> MHHHHHHGENLYFQGSGVEVIFYLSDREPLRLGSGEYTAEELCIRAAQACRISPLCHNLFALYDEN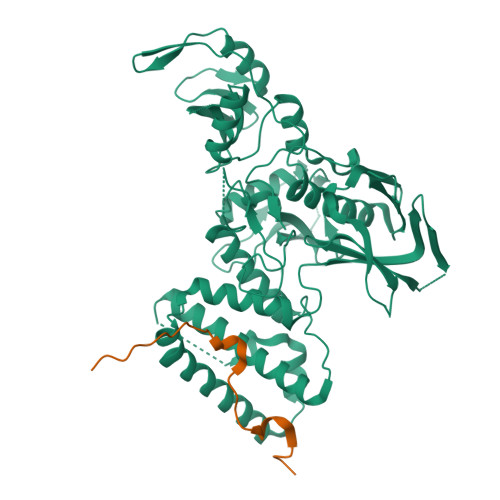TKLWYAPNRTITVDDKMSLRLHYRMRFYFTNWHGTNDNEQSVWRHSPKKQKNGYEKKKIPDATPLLDASSLEYLFAQGQYDLVKCLAPIRDPKTEQDGHDIENECLGMAVLAISHYAMMKKMQLPELPKDISYKRYIPETLNKSIRQRNLLTRMRINNVFKDFLKEFNNKTICDSSVSTHDLKVKYLATLETLTKHYGAEIFETSMLLISSENEMNWFHSNDGGNVLYYEVMVTGNLGIQWRHKPNVVSVEKEKNKLKRKKLENKDKKDEEKNKIREEWNNFSFFPEITHIVIKESVVSINKQDNKKMELKLSSHEEALSFVSLVDGYFRLTADAHHYLCTDVAPPLIVHNIQNGCHGPICTEYAINKLRQEGSEEGMYVLRWSCTDFDNILMTVTCFEKSEQVQGAQKQFKNFQIEVQKGRYSLHGSDRSFPSLGDLMSHLKKQILRTDNISFMLKRCCQPKPREISNLLVATKGNS;> GSKTLMGNPWFQRKKLPSVLLFKKPSPFIFISQRPSPETQDTIHPLDEEAFLK>[2x]MSYQGRARKFLESASIDVGDMVLVEKPDVTYEGMVLDRADDADDRHIVLKLENGYNIGVEISDARIELLEKGSEPRIELPPVEAAEDPELPDVSIISTGGTVASIIDYRTGAVHPAFTADDLLRANPELLDIANIRGRAVFNILSENMKPEYWVETARAVYGEIKDGADGVVVAHGTDTMHYTSAALSFMLRTPVPVVFTGAQRSSDRPSSDASLNIQCSVRAATSEIAEVTVCMHATMDDLSCHLHRGVKVRKMHTSRRDTFRSMNALPLAEVTPDGIKILEENYRKRGSDELELSDRVEERVAFIKSYPGISPDIIKWHLDEGYRGIVIEGTGLGHCPDTLIPVIGEAHDMGVPVAMTSQCLNGRVNMNVYSTGRRLLQAGVIPCDDMLPEVAYVKMCWVLGQTDDPEMAREMMRENIAGEINERTSIAYFRG;>MDWEKVGLKMGLEIHQQLDTESKLFCPCRTELTDSEPDHDIVRNLRPTQSELGKFDRAAFEEAMRKLHFHYENYHEETCLVEADEEPPHPLNPEALEIAVTIALLLNMRVVDEFHTMRKQVIDGSNTGGFQRTGLVATDGHLETPQGTVKIENLCLEEDAARRIRETGDGVVFRLDRLGIPLVEITTDPSMSDPQQLREVAYQIGQILRSTRVKRGLGTIRQDLNISIRDGARVEVKGVQDLDLIPEIVEREVKRQLSLVEIRDTLQERGAVVEDKIFDVSEVFADTESRIISSAESVLAVKLRGFDGLIGVEIQPGRRLGTEMADYAKKRGVSGIFHTDELPAYGITEEEVRGLRDAVGASQGDAVVMVAHERVTAENALREVIRRAEMAIQGVPEETRKALPDGNTQYLRPLPTSSRMYLETDIPLFRIEDDLLEGI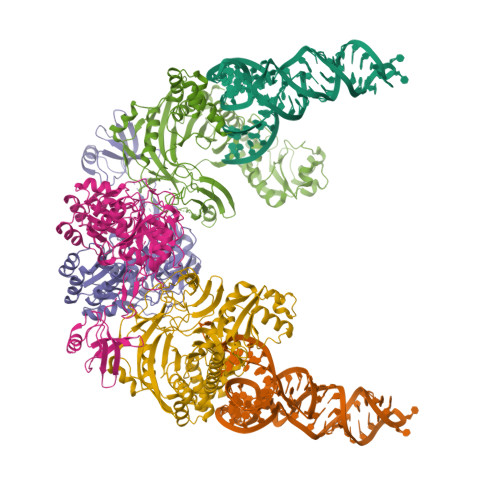RRNLPELPSEKKERIMRDYGLSEDLASQLVKRNLVDEFEALTEFRVDTTVIASLLAYTLRELRREGHDVDGLGLDELRDAIKLLEVGKISKDALRDIVACMADEGLAAEDAARKLNLLLLAEDEIESIIQEIVEGNLDMISERGMGAMGPLMGQAMGRLRGRADGKVVNRILREKIQERL[2x]> MYLSKVIIARAWSRDLYQLHQGLWHLFPNRPDAARDFLFHVEKRNTPEGCHVLLQSAQMPVSTAVATVIKTKQVEFQLQVGVPLYFRLRANPIKTILDNQKRLDSKGNIKRCRVPLIKEAEQIAWLQRKLGNAARVEDVHPISERPQYFSGDGKSGKIQTVCFEGVLTINDAPALIDLVQQGIGPA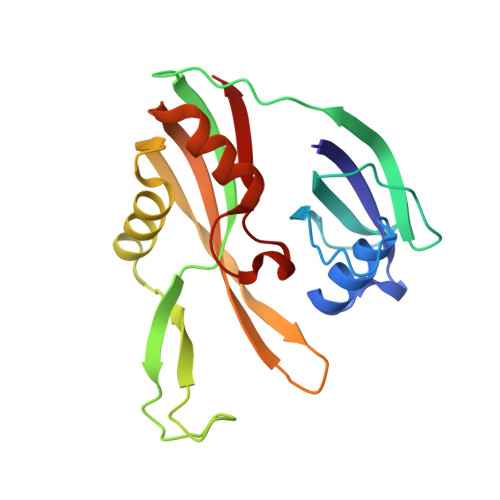KSMGCGLLSLAPL>GSHMAKEEIIWESLSVDVGSQGNPGIVEYKGVDTKTGEVLFEREPIPIGTNNMGEFLAIVHGLRYLKERNSRKPI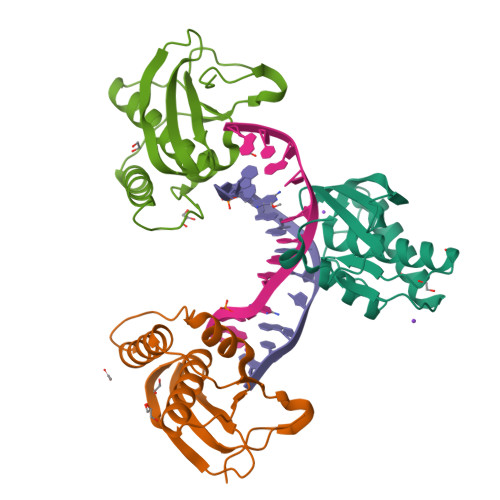YSNSQTAIKWVKDKKAKSTLVRNEETALIWKLVDEAEEWLNTHTYETPILKWQTDKWGEIKADYGRK[3x]N-[2-fluoro-6-(pyrrolidin-1-yl)phenyl]-N'-{3-[(2R)-1-(2-hydroxyethyl)-4-(7H-pyrrolo[2,3-d]pyrimidin-4-yl)piperazin-2-yl]phenyl}urea | C29 H33 F N8 O2 | 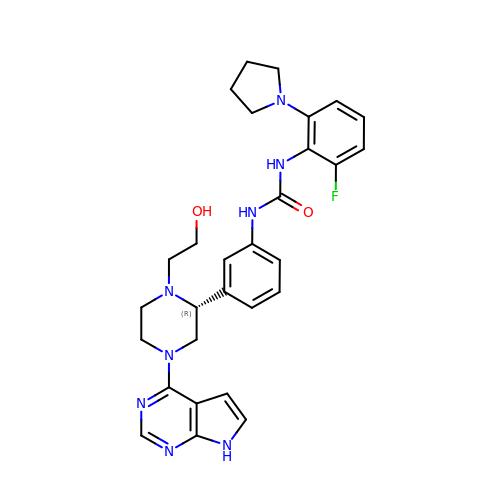ZJSNZHATZAWKIQ-VWLOTQADSA-N>MHHHHHHTMAAPVSTQLSQDELKKQAAWKAVEYVKSGMVVGLGTGSTAAFAVDRIGQLLKEGKLQNIVGVPTSIRTYEQALSLGIPLATLDEQPKLDVAIDGADEVDPNLDVVKGRGGALLREKM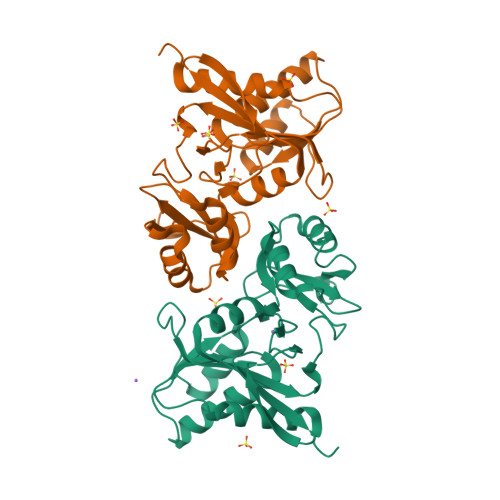VEMASAKFVCIVDDSKLVEGLGGSKLAMPVEIVQFCHKYTLQRLANLPEVKGCEAKLRMNGDKPYVTDNSNYIVDLYFQTPIKDSQAASKAILGLDGVVDHGLFLDMVDVCIIAGATGVTVQERPNPKKH[2x]(5R,6R,7R,8S)-6,7-dihydroxy-5-(hydroxymethyl)-2-(2-phenylethyl)-8-(propanoylamino)-5,6,7,8-tetrahydro-1H-imidazo[1,2-a]pyridin-4-ium 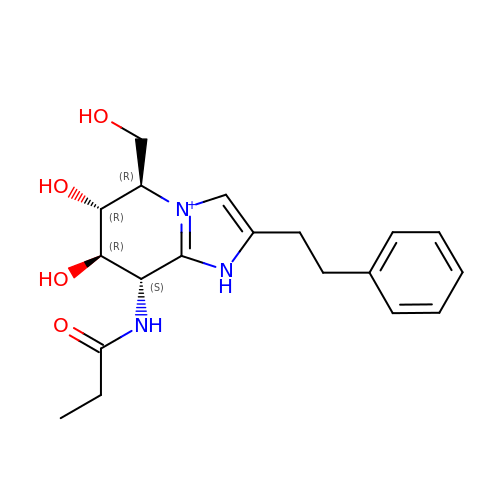| C19 H26 N3 O4 | QLPMCDAONBPCJU-VDHUWJSZSA-O> GPLGSMDDGSVSDIKRGRAARNAKLASIPVGFAGRAALGLGKRLTGKSKDEVTAELMEKAANQLFTVLGELKGGAMKVGQALSVMEAAIPDEFGEPYREALTKLQKDAPPLPASKVHRVLDGQLGTKWRERFSSFNDTPVASASIGQVHKAIWSDGREVAVKIQYPGADEALRADLKTMQRMVGVLKQLSPGADVQGVVDELVERTEMELDYRLEAANQRAFAKAYHDHPRFQVPHVVASAPKVVIQEWIEGVPMAEIIRHGTTEQRDLIGTLLAELTFDAPRRLGLMHGDAHPGNFMLLPDGRMGIIDFGAVAPMPGGFPIELGMTIRLAREKNYDLLLPTMEKAGLIQRGRQVSVREIDEMLRQYVEPIQVEVFHYTRKWLQKMTVSQIDRSVAQIRTARQMDLPAKLAIPMRVIASVGAILCQLDAHVPIKALSEELIPGFAEPDAIVV

In this study, we have identified a non-canonical ABC protein encoded by the rv3197 gene in M. tuberculosis, as a macrolide antibiotic binding protein (MABP-1), which confers inducible resistance to the macrolide family of antibiotics. MABP-1 adopts an unusual three-dimensional fold with a kinase-like domain and a linked accessory domain. MABP-1 is a homodimer with each subunit containing a bilobal kinase domain and an accessory domain. The accessory domain is indispensable for its function where it participates in dimerization of MABP-1 and in erythromycin binding.

The crystal structure of apo-MABP-1 was determined at 2.2 Å by single wavelength anomalous dispersion (SAD). According to a DALI search the kinase domain strongly resembles that of an ancient UbIB protein kinase (ADCK3). The accessory domain consists of six α-helices: α1–α4 helices (residues 1–120) and α6–α7 helices (residues 161–206). These regions are insertions that are not found in the canonical kinase structures. Crucially, the α1 and α2 helices in each subunit insert into the accessory domain of its adjoining subunit, resulting in an N-terminal domain-swapped dimer. The accessible surface area that is buried upon dimerization is extensive, at 2021 Å2 per subunit.>[6x]GHMVTRIENLENAKKLWDNANSMLEKGNISGYLKAANELHKFMKEKNLKEDDLRPELSDKTISPKGYAILQSLWGAASDYSRAAATLTESTVEPGLVSAVNKMSAFFMDCKLSPNERATPDPDFKVGKSKILVGIMQFIKDVADPTSKIWMHNTKALMNHKIAAIQKLERSNNVNCETLESVLSSKGENLSEYL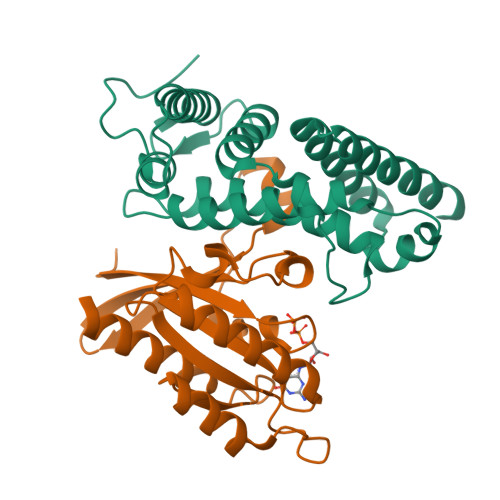SYK;>MAPEYDYLFKLLLIGDSGVGKSCLLLRFADDTYTESYISTIGVDFKIRTIELDGKTIKLQIWDTAGQERFRTITSSYYXGAHGIIVVYDVTDQESYANVKQWLQEIDRYASENVNKLLVGNKSDLTTKKVVDNTTAKEFADSLGIPFLETSAKNATNVEQAFMTMAAEIKKRMGHHHHHH[6x]>[4x]SNAMSAGKRVLVAGVGNRLMGDDGFGPRVVDL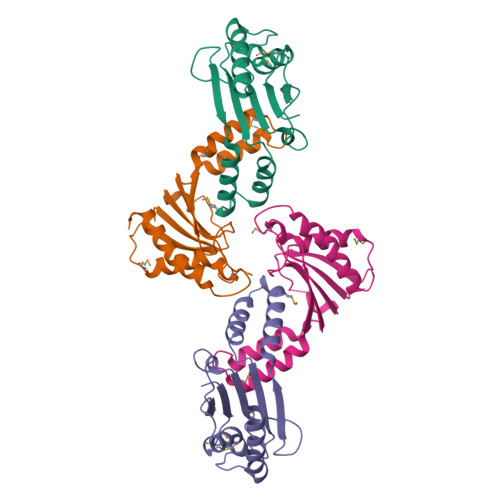LSSMSLPDYVDARDIGTAGITVATDLEDYEKVIFLDSVELEGPPGRLSKSILEVRGLDEDISQLARMTLHEVGLEGLLKFAKSIGVLPGEVTLIGCIPRSLKPSLELSEEVEAATHAAVDLVLEALGLE>[12x]GKVYKKVELVGTSEEGLEAAIQAALARARKTLRHLDWFEVKEIRG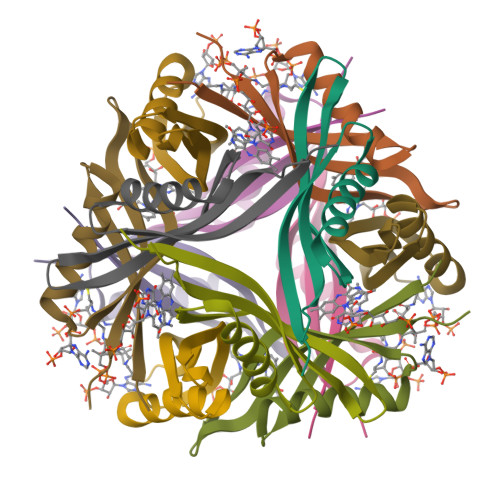TIGEAGVKEYQVVLEVGFRLEET> ADIYIPTLEEIKRTLQLAKDYSENVYFIYRIALESGVRLSEILKVLKEPERDICGND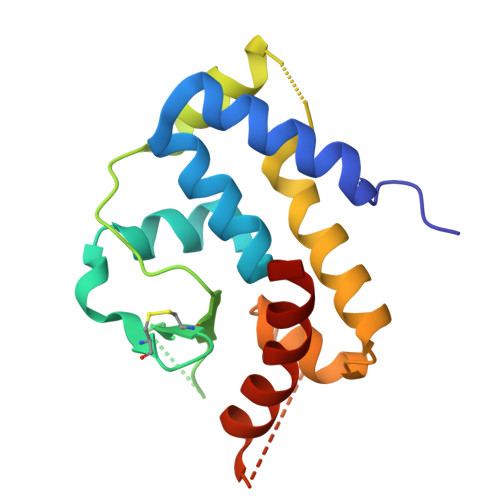VCYYPLSWTRGYKGVFYVFHITPLKRVEVTKWAIADFERRHKDAIAIKYFRKFVASKMAELSVPLDIIDFIQGRKPTRVLTQHYVSLFGIAKEQYKKYAEWLKGV>[3x]MNALLSNP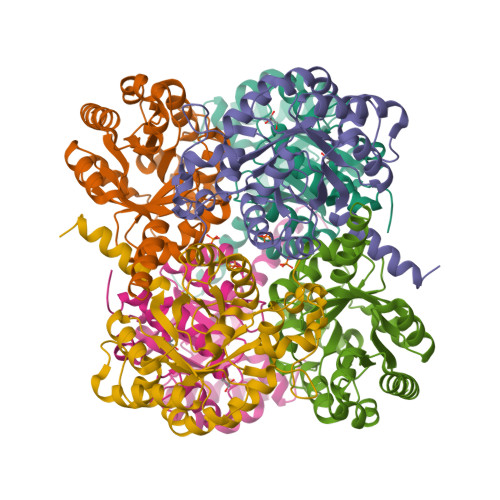FKERLRKGEVQIGLWLSSTTAYMAEIAATSGYDWLLIDGEHAPNTIQDLYHQLQAVAPYASQPVIRPVEGSKPLIKQVLDIGAQTLLIPMVDTAEQARQVVSATRYPPYGERGVGASVARAARWGRIENYMAQVNDSLCLLVQVESKTALDNLDEILDVEGIDGVFIGPADLSASLGYPDNAGHPEVQRIIETSIRRIRAAGKAAGFLAVAPDMAQQCLAWGANFVAVGVDTMLYSDALDQRLAMFKSGKNGPRIKGSY> ESTTVKMYEALPTGPGKEVGTVVISEAPGGLHFKVNMEKLTPGYHGFHVHENPSCAPGEKDGKIVPALAAGGHYDPGNTHHHLGPEGDGHMGDLPRLSANADGKVSETVVAPHLKKLAEIKQRSLMVHVGGDNYSDKPE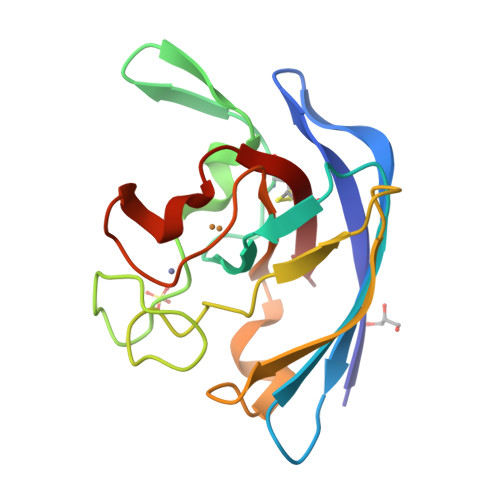PLGGGGARFACGVIE>[2x]APHMFSIRKIITISDYVTMLNIITGLLAILLNSFS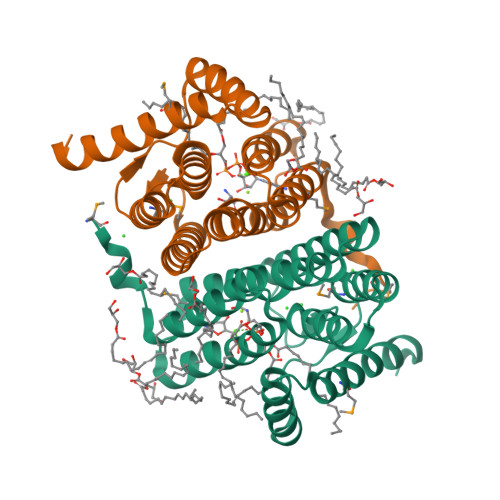LIYLSIIFDSLDGYVARKTGTVSDFGAELDSISDVVSFGVAPAYLLYNNFESNLALISAIIFCLCGALRLARFGILNVKGFIGLPIPAGALLLVGFCQLINSYLINSILAILIGLLMISDIKYPKYPNKIFIYIFAVSLCLAIVGIPHFALMLCLIYAIYGIIKYIRGD> MAELLTLARPYAKAAFAYASEQGATDNWSNALQVLSAAVQDEAFSAYLNRPELTPAEQVKLFAKVLGEDQSQAVSNFLTLLADNDRLVLLPEIAAEYEQ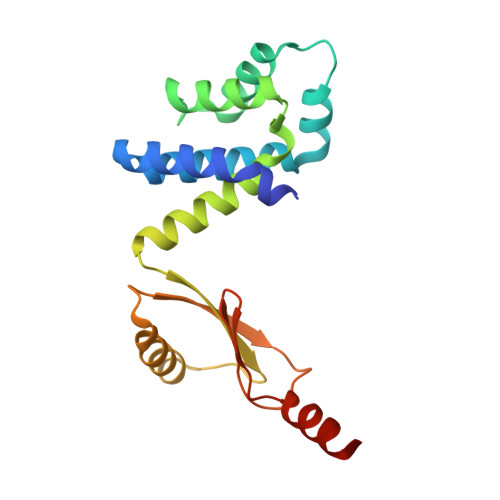LKSQNNNNVDVVIESAFPLTAEQEQLLKSALEKRFNSTVTVSVEVKPELIAGVVIRAGDQVIDDSALNKLEKMRTRLLA> MSLQLLRNTRIFVSTVKTGHDTTNTQEILVQDDISWGQDSNSTDITVNEAGPRPTRGSKRFNDSLNAAEWSFSTYILPYEDTTTGKQIVPDYMLWHALSS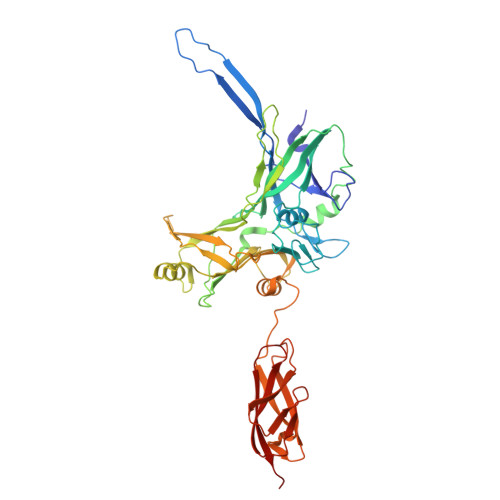GKAIDLDGDTGAHNNATNFMVNFKDNAYHELAMLHIYILTDNAWSYIDSCQINQAEVNVDIEDIGRVTWSGNGNQLIPLDEQPFDPDALGIDDETYMTIQSSYIKNKLTILKIKDMDSDKEYDIPITGGTFTINNNITYLTPNIMSRVNIPIGSFTGAFELTGSLTAYLNDKSLGSMELYKDLVRTLKVVNRFEIALILGGEYDDERPAAVLVAKQAHVNIPTIETDDVLGTSVEFKAIPTDLDTGDEGYLGFSNKYTKTTVANLIATGDGAETPPILVESITVKSAADATSVTNSDTLQMSVEVTPPEATNTAVTWSISSGDAATIDAESGLLTADVSKTGEVIVKAVAKDGSGVEGTKTITVSAGE>[5x]SNAMEKLIVGKSLEHQLDTVIKELAPAGNISYAVLQFDDEEEPTLIAARGENTVHSSASLIKVLIMEYVFHLARTEQLDINDTVPLSRTPRVEGGGALQELVGKHSFTYLELCRLMMVLSDNIATNLLITVLGMENINA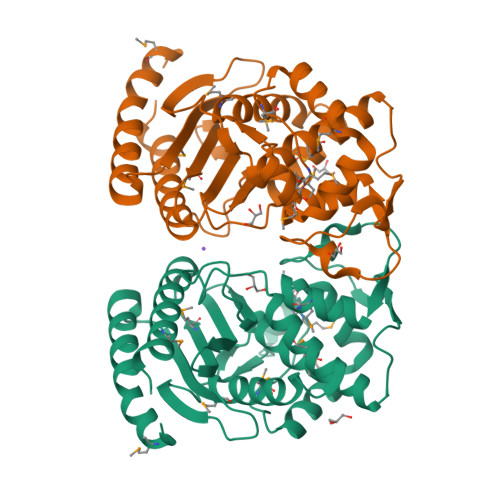RAEKLGVDEMELNRMMMDFNALAEGRDNHITAMSLARLYKHIFECRDRDVYGREMWNILGRQQFRDILPFYWGEGIRFHHKTGSLDRVEHDGGVIETFRGHFCFILLMSDIDNDRGKELGAQVGRIMKEFVEEALP> GSPEFMDDIFTQCREGNAVAVRLWLDNTENDLNQGDDHG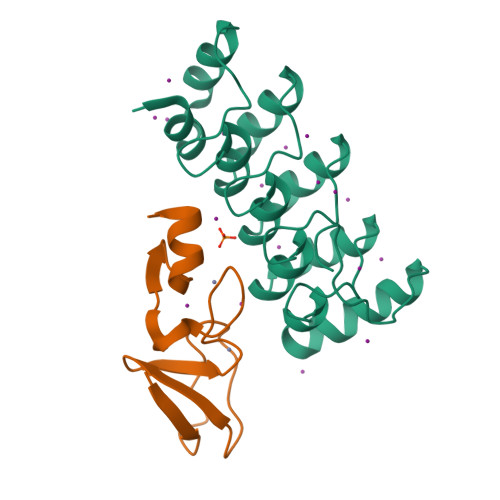FSPLHWACREGRSAVVEMLIMRGARINVMNRGDDTPLHLAASHGHRDIVQKLLQYKADINAVNEHGNVPLHYACFWGQDQVAEDLVANGALVSICNKYGEMPVDKAKAPLRELLRERAEKMGQNLNRIPYKDTFWKGTTR;> SENLYFQGSASATCERCKGGFAPAEKIVNSNGELYHEQCFVCAQCFQQFPEGLFYEFEGRKYCEHDFQMLFA> ADTATVAPIPDAIAKHQGQIKIAVIRNLGSDDNTTQFLSGVLKEGKKLGFKVDTFLSNGDDARFQDFVNQAISQKYDGIILSQGRDPYSTELVKRIVANGIAVSVFDTAIQGDIPGLTVTQQDDASLTNESFGQLVKDFNGKANIIKLWVAGFPPMERRQAAYQALLKQNPGITELESIGAVSSDVQGDTANKVGAVLAKYPKGKIDAIWGTWDAFTQGAYKALQENGRTEIKLYSIDISNQDLQLMREANS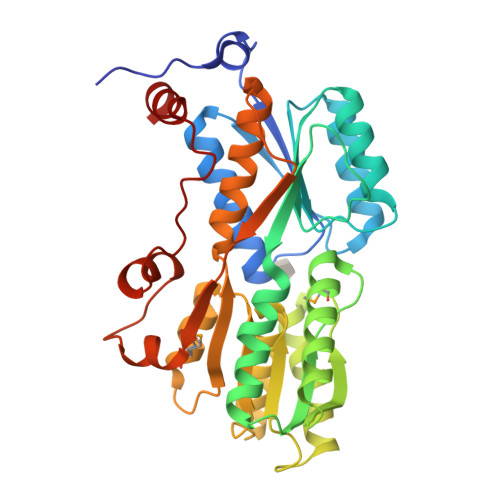PWKVSVAVDPKLIGAVNLRLVAKKIAGEETPASYEFRAASIPQALLVSQPGPVNVSGLSKIIPGWGQSDDFNSPWFATLAAKNGQ>TGATCA[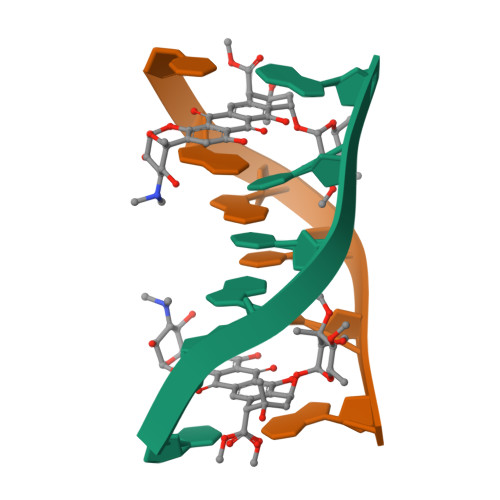2x]> DQSSCCDKEIIKDVSELTGIISYNTEVKRWYISVSDANSYDNVTLYFPCNLDSKYMKEKEKVIFSGQISKSTLKITLPAGTTSYCIN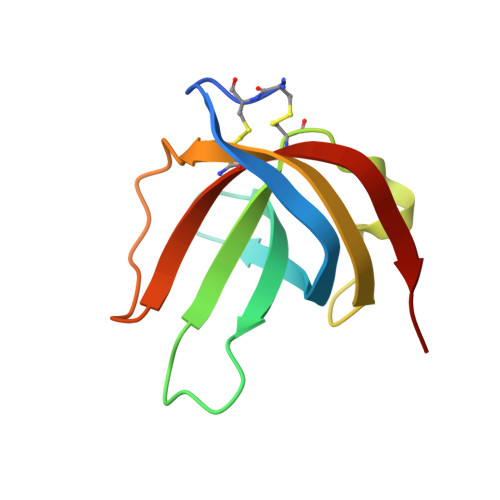LMSINKIN> SPQPLEQIKLSESQLSGRVGMIEMDLASGRTLTAWRADERFPMMSTFKVVLCGAVLARVDAGDEQLERKIHYRQQDLVDYSPVSEKHLADGMTVGELCAAAITMSDNSAANLLLATVGGPAGLTAFLRQIGDNVTRLDRWETELNEALPGDARDTTTPASMAATLRKLLTSQRLSARSQRQLLQWMVDDRVAGPLIRSVLPAGWFIADKTGAGERGARGIVALLGPNNKAERIVVIYLRDTPASMAERNQQ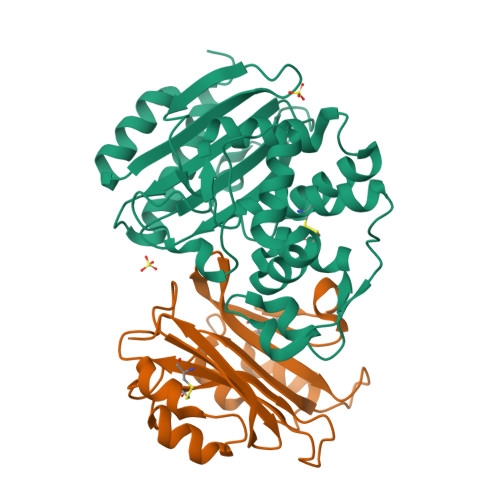IAGIGAALIEHWQR;> AGVMTGAKFTQIQFGMTRQQVLDIAGAENCETGGSFGDSIHCRGHAAGDYYAYATFGFTSAAADAKVDSKSQMKLLAPSAPTLTLAKFNQVTVGMTRAQVLATVGQGSCTTWSEYYPAYPSTAGVTLSLSCFDVDGYSSTGFYRGSAHLWFTDGVLQGKRQWDLV> ATFLIWPIYPKIEANEKATAVWLQNTGKTDAMVQIRVFKWNQDGLKDNYSEQSEIIPSPPVAKIKAGEKHMLRLTKSVNLPDGKEQSYRLIVDELPIRLSDGNEQDASKVSFQMRYSIPLFAYGKGIGSGLTEESQKLNAKNALAKPVLQWSVRNNQQGQSELYLKNNGQKFARLSALKTSKTGNDISLGKAAFGYVLSNSTVKFAIDQSTAHELAKTSKIYGVDSSGIKQELIEITKMEDPS;> AVTHHHHHHSTGCTVGGSQTEGNMNKFGTLNFGKTSGTWNNVLTAEVASAATGGNISVTCDGTDPVDFTVAIDGGERTDRTLKNTASADVVAYNVYRDAARTNLYVVNQPQQFTTVSGQATAVPIFGAIAPNTGTPKAQGDYKDTLLVTVNF

The major class of these adhesive pili (or fimbriae) is assembled via the classical, alternative and archaic chaperone-usher (CU) pathways. The biogenesis of CU fibres requires a periplasmic chaperone and outer membrane assembly platform termed the usher. Here, we report atomic-resolution insight into the structure and biogenesis of Acinetobacter baumannii Csu and Escherichia coli ECP pili assembled via the archaic and alternative pathways, respectively, whilst also highlighting some important deviations from the classical assembly mechanism. The non-classical chaperones, unlike their classical counterparts, maintain subunits in a substantially unfolded state by utilising a register-shifted DSC and a distinct subunit C-terminal carboxylate anchor.

Archaic Csu pili mediate the formation of Acinetobacter baumannii biofilms, which contribute to high rates of nosocomial infections. This pilus is formed from four subunits, namely CsuA/B, CsuA, CsuB, and CsuE, and is assembled using the CsuC-CsuD chaperone-usher secretion machinery. To gain insight into the structure and assembly of archaic CU pili, we determined the crystal structure of a CsuC-CsuA/B pre-assembly complex, composed of His6-CsuA/B and CsuC (to avoid polymerisation). Crystals were readily obtained in spacegroup P6422 and the structure was solved using Se-SAD phasing to a resolution of 2.4 Å. The CsuC chaperone has a canonical Ig-like fold with two 7-stranded β sandwich domains (D1 and D2) oriented at ∼90° angle. Whilst the refinement statistics for the structure of the CsuC-CsuA/B complex are good, approximately 40% of the CsuA/B sequence was not evident in electron density maps, whilst another 7% has very poor electron density (Cα atom B-factors higher than 80 A2). The remaining structure of the CsuA/B subunit reveals a double β-sheet sandwich comprising strands A, B, and E (β-sheet 1) and C and F (β-sheet 2) and β-strand D, which switches between the sheets. Nevertheless, the ordered part of CsuA/B provides sufficient information to conclude that, as with classical systems this pilin has the incomplete Ig-like fold in a six-stranded β-sandwich, in which the absent 7th strand (G) leaves a large hydrophobic cleft. CsuA/B interacts predominantly with D1 of the chaperone CsuC via edge strands to form a closed “super-barrel” with a common core. Four large hydrophobic residues from the chaperone G1 strand (Val110, Phe112, Met114, Tyr116) are donated to the subunit to compensate for the missing G strand. The C-terminal carboxylate of Phe152 interacts with two highly conserved residues of CsuC.>MERLDIFGVPIDRVTMIQAVDILNNFLQENRLHIVATPNAEIVMMAQKDKEYMEILNNTDLNVPDGSGIVFASKVFKKPLPERVAGFDLMLEFIKGISSKGVKIYLLGAAAQVAEQARANLEKLYPGVKIVGTHHGYFTEEEENKIIEEINNKGAEVLFVALGAPKQEKWIYKNKDKLKVKIAMGVGGSFDVIAGKVKRAPYEYRKLGQEWKYRLEKEPWRYKRMMA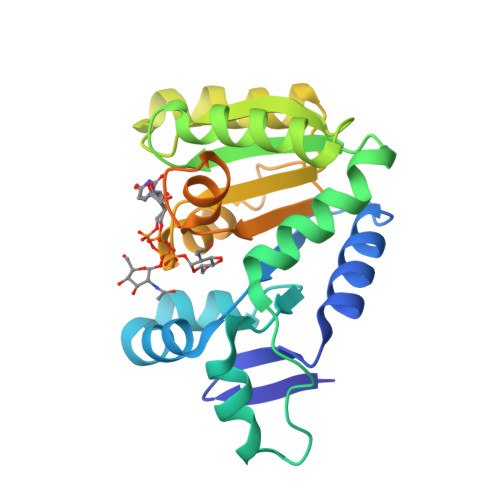LPKFAIKVLLHKREVVR[3x]>MASVHGTTYELLRRQGIDTVFGNPGSNELPFLKDFPEDFRYILALQEACVVGIADGYAQASRKPAFINLHSAAGTGNAMGALSNAWNSHSPLIVTAGQQTRAMIGVEALLTNVDAANLPRPLVKWSYEPASAAEVPHAMSRAIHMASMAPQGPVYLSVPYDDWDKDADPQSHHLFDRHVSSSVRLNDQDLDILVKALNSASNPAIVLGPDVDAANANADCVMLAERLKAPVWVAPSAPRCPFPTRHPCFRGLMPAGIAAISQLLEGHDVVLVIGAPVFRYHQYDPGQYLKPGTRLISVTCDPLEAARAPMGDAIVADIGAMASALANLVEESSRQ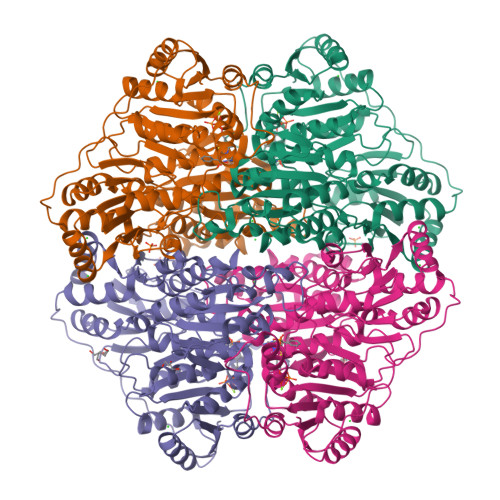LPTAAPEPAKVDQDAGRLHPETVFDTLNDMAPENAIYLNESTSTTAQMWQRLNMRNPGSYYFCAAGGLGFALPAAIGVQLAEPERQVIAVIGDGSANYSISALWTAAQYNIPTIFVIMNNGTYGALRWFAGVLEAENVPGLDVPGIDFRALAKGYGVQALKADNLEQLKGSLQEALSAKGPVLIEVSTVSPVKHHHHHH[4x]>[3x]GSKKIFKPEELRQALMPTLEALYRQDPESLPFRQPVDPQLLGIPDYFDIVKNPMD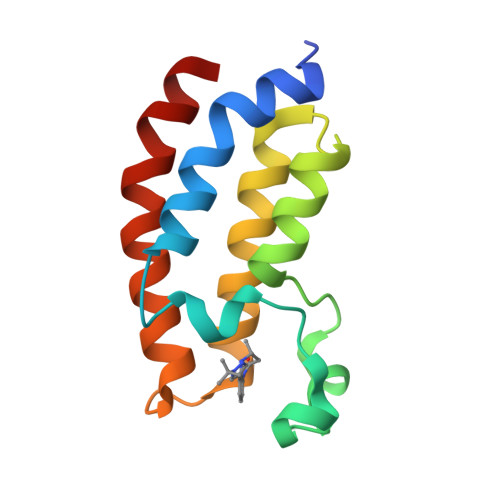LSTIKRKLDTGQYQEPWQYVDDVWLMFNNAWLYNRKTSRVYKFCSKLAEVFEQEIDPVMQSLG> GAGCAGACTTG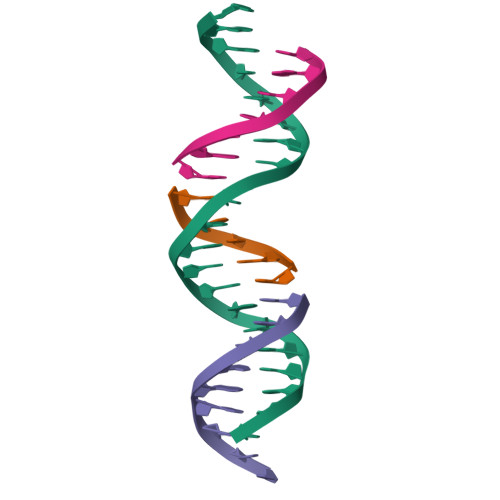ACAGCACTCA;> TGTCA;> TCTGAGTGC;> AGTCTGC> GAEPREPADGQALLRLVVELVQELRKHHSAEHKGLQLLGRDYALGRAEAAGLGPSPEQRVEIVPRDLRMKDKFLKHLTGPLYFSPKCSKHFHRLYHNTRDCTIPAYYKRCARLLTRL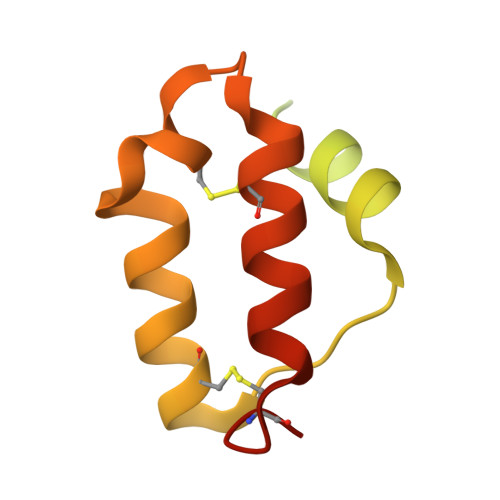AVSPVCMEDKQ6-ethyl-5-{(3R)-3-[3-methoxy-5-(morpholin-4-yl)phenyl]but-1-yn-1-yl}pyrimidine-2,4-diamine | C21 H27 N5 O2 | 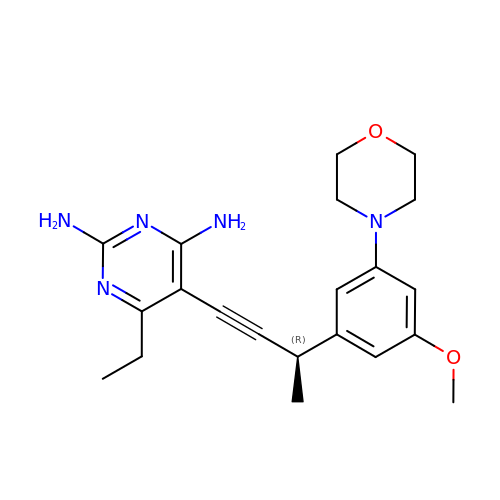DNZHKQMESCYJCG-AWEZNQCLSA-N>APVWGCASTRGRSAEMEDASAAVPRFADVPVRLLASRRDLDALGLDADALRLPAHLFGVFDGHGGAEVANYCRERIHVVLSAALARLGKNLGEMGEVDMKEHWDDVFTKCFQRVDDEVSGRVTRVVNGGGEVRSEPVTAENVGSTAVVALVCSSHVVVANCGDSRIVLCRGKEPVALSIDHKPDRKDERARIEAQGGKVIQWNGYRVSG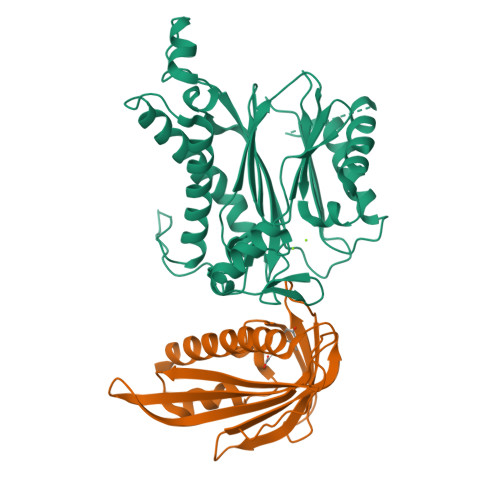WLAMSRSIGDRYLKPFVIPKPEVMVVPRAKDDDCLILASDGLWDVVSNEEACKVARRQILLWHKNNGAASPLSDEGEGSTDPAAQAAADYLMRLALKKGSEDNITVIVVDLKPRKKLKN[2x];>ETEYVRRFHRHEPRDHQCSSAVAKHIKAPVHLVWSLVRRFDQPQLFKPFVSRCEMKGNIEIGSVREVNVKSGLPATRSTERLELLDDNEHILSVRFVGGDHRLKNYSSILTVHPEVIDGRPGTLVIESFVVDVPEGNTKDETCYFVEALLKCNLKSLAEVSERLVVKDQTEPLDR[2x]>DTMKVINDPIHGHIELHPLLVRIIDTPQFQRLRYIKQLGGGYYVFPGASHNRFEHSLGVGYLAGCLVHALGEKQPELQISERDVLCVQIAGLCRNLGHGPFSHMFDGRFIPLARPEVKWTHEQGSVMMFEHLINSNGIKPVMEQYGLIPEEDICFIKEQIVGPLESPVEDSLWPYKGRPENKSFLYEIVSNKRNGIDVDKWDYFARDCHHLGIQNNFDYKRFIKFARVCEVDNELRICARDKEVGNLYDMFHTRNSLHRRAYQHKVGNIIDTMITDAFLKADDYIEITGAGGKKYRISTAIDDMEAYTKLTDNIFLEILYSTDPKLKDAREIL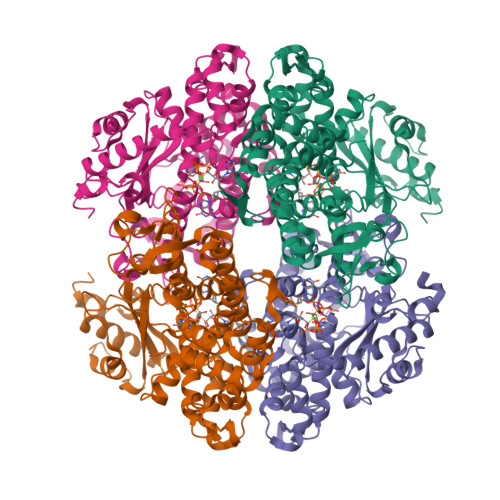KQIEYRNLFKYVGETQPTGQIKIKREDYESLPKEVASAKPKVLLDVKLKAEDFIVDVINMDYGMQEKNPIDHVSFYCKTAPNRAIRITKNQVSQLLPEKFAEQLIRVYCKKVDRKSLYAARQYFVQWCADRNFTKPQDGDVIAPLIVPQKKEWNDSTSVQNPTRLREASKSRVQLFKDDPM[4x]> LESHMTPKDDEFYQQWQLKYPKLILREASSVSEELHKEVQEAFLTLHKHGCLFRDLVRIQGKDLLTP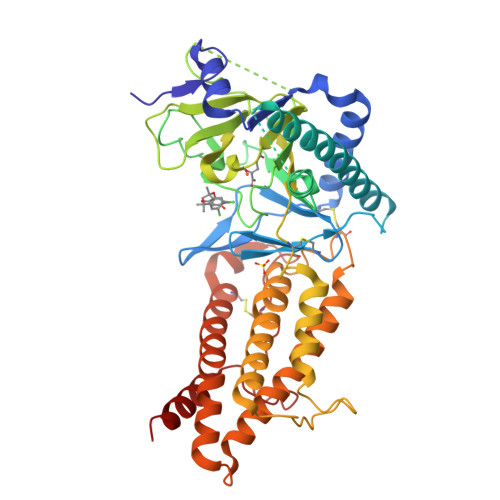VSRILIGNPGCTYKYLNTRLFTVPWPVKGSNIKHTEAEIAAACETFLKLNDYLQIETIQALEELAAKEKANEDAVPLCMSADFPRVGMGSSYNGQDEVDIKSRAAYNVTLLNFMDPQKMPYLKEEPYFGMGKMAVSWHHDENLVDRSAVAVYSYSCEGPEEESEDDSHLEGRDPDIWHVGFKISWDIETPGLAIPLHQGDCYFMLDDLNATHQHCVLAGSQPRFSSTHRVAECSTGTLDYILQRCQLALQNVCDDVDNDDVSLKSFEPAVLKQGEEIHNEVEFEWLRQFWFQGNRYRKCTDWWCQPMAQLEALWKKMEGVTNAVLHEVKREGLPVEQRNEILTAILASLTARQNLRREWHARCQSRIARTLPADQKPECRPYWEKDDASMPLPFDLTDIVSELRGQLLE>MRGSMIKIIKNAKVFSPEYIGKKDVIFYHKVIHVGEGVNTSVLPFEHEIYDANGLLLLPGLIDPHVHITGGGGEGGFETRTPELKISDCIRSGVTTVVGCLGTDGITRSLENLYAKAKSLESEGLNTFIYTGSYRVPPVTFTGSIMRDIVLIDKVIGVGEIAISDHRSSQPTLEEILRIVADIRVGGMISGKAGIVNFHVGSGKRGIEYLFDIIEKTEIPIQHLYPTHMSRSRKLFEQGLEFAKRGGTIDLTALQPKDAEFVRAEFTTIDAICEAYENGLLDNVTISSDGQGSLPKFDDNGNFVGLDVGSVSAVWYTIRKVLEKGLPLAEVLKISTTNPARVFKLNKGKIAKGQDADFILVDEQSFEIVSVISKGEFLMKDGVMKNLNFEF[4x]

In the present study, we functionally characterized the hyperthermophilic M38 β-aspartyl peptidase FiBAP, a protein repair enzyme involved in hydrolysis of isoAsp residue-containing peptides in F. islandicum AW-1. The overall structure of each monomer can be divided into two distinct domains; an N-terminal β-sandwich domain (M1–G56; G344–E386) and a C-terminal catalytic domain (L57–K343), that are mainly involved in dimerization and catalysis, respectively. The catalytic domain at the C-terminus of the molecule folds into a (β/α)8 triosephosphate isomerase (TIM)-barrel motif.

Crystal structures of the ligand-free form of FiBAP and the ligand-bound form bound with N-carbobenzoxy-β-Asp-Leu (Cbz-β-DL) as a substrate analog were determined at resolutions of 2.6 and 2.7 Å, respectively. Cbz-β-DL-free and -bound structures belonged to I422 and P2212 space groups, with one and four subunits in the asymmetric unit, respectively. Intriguingly, the ligand-bound model included obvious electron density corresponding to loop P290–L302 between β14 and β15, which might have been stabilized upon ligand binding. Remarkably, the Cbz-β-DL-bound FiBAP structure aligned with the ligand-free model with an RMSD of 0.433 Å, despite the good superimposition of the structural elements. Such an unusually high RMSD value might be ascribed to the transformation of the missing loop (P290–L302) in the ligand-free structure into two stable antiparallel β-sheets (β14 and β15) in the ligand-bound structure. Since this stabilized loop is located next to the substrate-binding site, it might function as a gate for substrate entry and/or product release. Intriguingly, the crystal structure of FiBAP bound to Cbz-β-DL included distinct electron density only for the β-DL moiety lacking carbamazepine (Cbz) in the active site. There is no significant perturbation in the coordination of the binuclear zinc center in the Cbz-β-DL-bound FiBAP structure. However, structural comparison of the residues around the ligand-binding site reveals subtle changes of ~1 Å in the side-chain conformations of some residues (G68, E70, Y130, R163, R227, and S289) between Cbz-β-DL-free and -bound forms. Residues such as Y130, G68, and S289 are placed closer to the ligand than those in the ligand-free structure, thereby assisting coordination and stabilization, while R227 and R163 move away to provide space for ligand binding. The other surrounding residues that help to stabilize the bound Cbz-β-DL are the amino groups of main-chain residues S289 and G68, while T99 interacts with O04 and O05 atoms of the side-chain of the Asp residue of β-aspartyl leucine to stabilize the N-terminus of the dipeptide during substrate recognition.> MSNMMYNMKWQEAINDLMEQVTLEYLPLEQNEQQLGMKYKRDSSEWFHFWATLYIKYIDIYKKLEDCYDQLVHPQKRVLLKEMLENVIVRLCETKSQVVKYNTQYDATYKSDYPNLDELVMDLKLTPDCLDIPIPRYFREEDKKRLDERNQILDALLLEYTDTKEPQEEQYEDQNTLQADMDTAIRIIQRYERGRQGIERANLAKILKKEEEKKLERQKKLAEGTEIGEETEKDDAALVIKKYWRGYKSRKLVQDIREEELLFLGMKKVVEDPTLPESQYKQAQNKRQKMKYIQEEHEQEFNDEIENLKRLVKGNEGPDILDKMRAERREWIMRELEKNEFKEAPQDPSEFYNQQVMDPEQQAAEAAKAAEEAKKKGAAKKDDKKKKGKPSELDEFLENNKPTGPSPIVLKLQEQIEKHSGEWSKRDETNNFEQKHETELAKMLIKPVVEEQIKQQVDEMIAEELDIVRLRYDIKKKKQKKPPRPRNKGKNKKKFPGDSSNKGRDPKDILAGLVEKRVAKKLIPASLMDLKGEQNVLGKIQEIQADENLKKTEALTDAKLKKAQLEEPSTKMPDPSIAQIRQIIAEYIAFPLGSKYAKEKLDKMNYFFFMGPRGSGKTLAVRALAHECNAIVLDISPSNIDGQYTDKKQIDGMINSAFKVAKEFQPAIIYCEDFEYIFGQAKKKKSQVNPLFAKMKKPLMDFKKGKFFEPEDRVVFIGSTNRPWDCSQKEIKSFFDKKIYFPFPNYGTRMLLFKTFLEQKKVPLPDNFPINTIAHITEGWSAGSFKMAIDRVFTERRLQKINEEQIKLSEFIGPLSNVPFTSKEEFKEFKK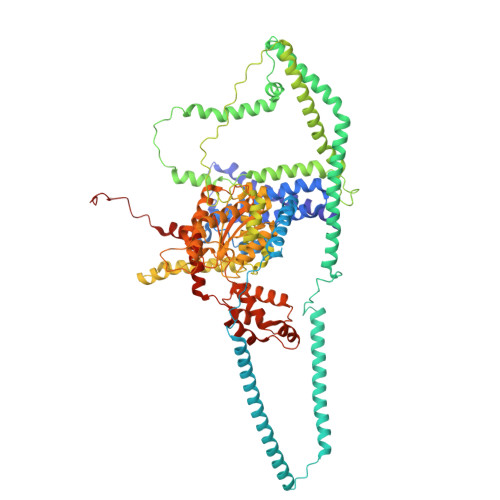FNQVVTGLQANYEAKKAPADDQKGDKNKKKK The universal N6-threonylcarbamoyladenosine (t6A) at position 37 of tRNAs is one of the core post-transcriptional modifications that are needed for promoting translational fidelity. In bacteria, TsaC uses L-threonine, bicarbonate, and ATP to generate an intermediate threonylcarbamoyladenylate (TC-AMP), of which the TC moiety is transferred to N6 atom of tRNA A37 to generate t6A by TsaD with the support of TsaB and TsaE. TsaD and TsaB form a TsaDB dimer to which tRNA and TsaE are competitively bound. In this study, we reconstituted tRNA t6A biosynthesis using TsaC, TsaD, TsaB, and TsaE from Aquifex aeolicus and determined crystal structures of apo-form and ADP-bound form of TsaD2B2 tetramer.

Therefore, we resolved a crystal structure of A. aeolicus TsaD–TsaB in complex with ADP and Fe2+ and a crystal structure of A. aeolicus TsaD–TsaB in complex with Fe2+. In both crystals, the asymmetrical unit contains a single TsaD and TsaB. α2 and α3 from TsaD and α1 and α2 from TsaB interact to form a typical “helical bundle” interacting interface of TsaDB dimer, which conforms to those of E. coli and T. maritima TsaDB dimers. Two TsaDB dimers from symmetrical units further interact and form a TsaD2B2 tetramer. Crystal structures of A. aeolicus and T. maritima TsaD2B2 tetramer exhibit that two β3s of TsaB form two antiparallel β-strands that mainly support the dimerization of TsaDB. The dimerization interface also involves ionic bonds and hydrogen bonds between α3 and α6 (in A. aeolicus TsaD2B2) and ionic bonds between α1s (in T. maritima TsaD2B2). Our structures captured an apo-form of TsaDB and an ADP-bound form of TsaDB, which are perfectly superimposed with an RMSD value of 0.18 Å over 4017 atoms. In our crystal structure of A. aeolicus TsaDB, the helical hairpin α1–α2 (Ser31–Glu50) of TsaD simultaneously contacts the connecting loop of α6 and α7 of TsaD and the C-terminal tail of TsaB, and adopts a conformation that prevents anticodon stem loop of tRNA from docking into the t6A-catalytic site of TsaD. Structural juxtaposition of A. aeolicus TsaB, T. maritima TsaB, and E. coli TsaB exhibit that A. aeolicus TsaB adopts a conserved fold of the N-subdomain and varied fold of the C-subdomain. A. aeolicus TsaB is composed of more long-range unstructured regions (with well-defined electron densities) between β7 and α5. In t6A-catalytic center of A. aeolicus TsaD, we identified an oxidized state of Cys10 (CSO10), which is in range of van der Waals force contact of the TC-moiety of TC-AMP (about 5 Å).

> MRTLAVETSCDETALAIYDDQKGVLGNVILSQAVVHSPFGGVVPELSAREHTRNILPIFDRLLKESRINLEEIDFISFTLTPGLILSLVVGVAFAKALAYEYRKPLVPVHHLEGHIYSVFLEKKVEYPFLALIISGGHTDLYLVRDFGRYDFLGGTLDDAVGEAYDKVAKMLGLGYPGGPIIDRLAKEGKKLYPLPKPLMEEGNLNFSFSGLKTAILNLLKKEKNVRKEDIAYSFQETVVEILLEKSLWAMKKTGIKRLVVVGGVSANSRLREVFKKASQEYGFELYIPHPSLSTDNALMIAYAGMERFKRGVVAPLDVNPQPNIPLEEFGRIWT;> MKILSIDTSFSFINFSVIEEEKVTFLHYLKSNKKTLELLPKIFEELCIRPENFDAFAVSVGVGYLTSLRIGVTFVKTWAYTLGKPVVSYKNLELLAKKTPVPFPKIPYLKVGSNVFYQIFEESSSSEVKVFKGEELRGYGISLKEFEDIKLGEKQFFHDIFPFSAYGGIYAYEFLKENPEGENVFEIEPIYVKPPYHVKD>[2x]ASTQGISEDLYNRLVEMATISQAAYADLCNIPSTIIKGEKIYNAQTDINGWILRDDTSKEIITVFRGTGSDTNLQLDTNYTLTPFDTLPQCNDCEVHGGYYIGWISVQDQVESLVKQQASQYPDYALTVTGHSLGASMAALTAAQLSATYDNVRLYTFGEPRSGNQAFASYMNDAFQVSSPETTQYFRVTHSNDGIPNLPPAEQGYAHGGVEYWSVDPYSAQ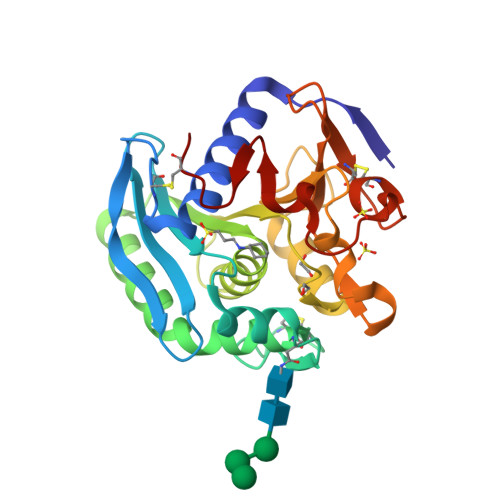NTFVCTGDEVQCCEAQGGQGVNDAHTTYFGMTSGACTW>SNAMGKVLSSSKEAAKLIHDGDTLIAGGFGLCGIPEQLILSIRDQGVKDLTVVSNNCGVDDWGLGLLLANKQIKKMIASYVGENKIFERQFLSGELEVELVPQGTLAERIRAGGAGIPGFYTATGVGTSIAEGKEHKTFGGRTYVLERGITGDVAIVKAWKADTMGNLIFRKTARNFNPIAAMAGKITIAEAEEIVEAGELDPDHIHTPGIYVQHVVLGASQEKRIEKRTVQQASGKGEAK[2x];>[2x]SNAMKEARKRMVKRAVQEIKDGMNVNLGIGMPTLVANEIPDGVHVMLQSENGLLGIGPYPLEGTEDADLINAGKETITEVTGASYFDSAESFAMIRGGHIDLAILGGMEVSEQGDLANWMIPGKMVKGMGGAMDLVNGAKRIVVIMEHVNKHGESKVKKTCSLPLTGQKVVHRLITDLAVFDFVNGRMTLTELQDGVTIEEVYEKT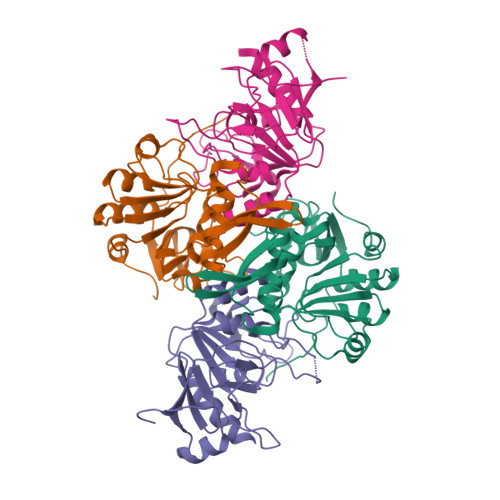EADFAVSQSVLNS> STYADYFSAWDKWEKQALPGEERDEAVSRLKECLINNSDELRLD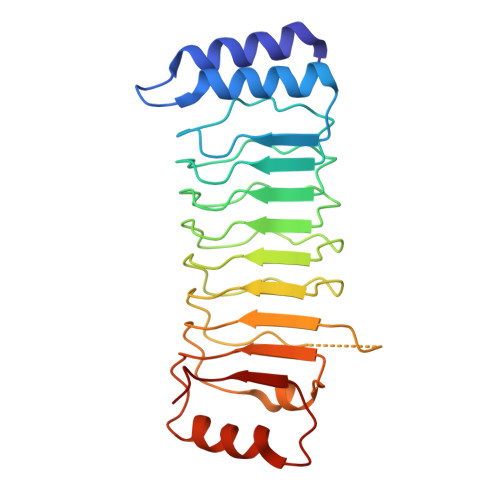RLNLSSLPDNLPAQITLLNVSYNQLTNLPELPVTLKKLYSASNKLSELPVLPPALESLQVQHNELENLPALPDSLLTMNISYNEIVSLPSLPQALKNLRATRNFLTELPAFSEGNNPVVREYFFDRNQISHIPESILNLRNECSIHISDNPLSSHALPALQRLTSSPDYHGPRIYFSMSD>MAPAEILNGKEISAQIRARLKNQVTQLKEQVPGFTPRLAILQVGNRDDSNLYINVKLKAAEEIGIKATHIKLPRTTTESEVMKYITSLNEDSTVHGFLVQLPLDSENSINTEEVINAIAPEKDVDGLTSINAGRLARGDLNDCFIPCTPKGCLELIKETGVPIAGRHAVVVGRSKIVGAPMHDLLLWNNATVTTCHSKTAHLDEEVNKGDILVVATGQPEMVKGEWIKPGAIVIDCGINYVPDDKKPNGRKVVGDVAYDEAKERASFITPVPGGVGPMTVAMLMQSTVESAKRFLEKFKPGLEHHHHHH[4x]

Methylenetetrahydrofolate dehydrogenase/cyclohydrolase 2 (MTHFD2) is a bifunctional metabolic enzyme found in mitochondria, exhibiting both dehydrogenase and cyclohydrolase catalytic activities. In one-carbon metabolism, MTHFD2 converts 5, 10-methylene tetrahydrofolate (5,10-CH2-THF) to 10-formyl tetrahydrofolate (10-CHO-THF) in mitochondria, thereby regulating the production of NADH, purines, and pyrimidines. An isozyme, methylenetetrahydrofolate dehydrogenase, cyclohydrolase and formyltetrahydrofolate synthetase 1 (MTHFD1), performs similar catalytic reactions to MTHFD2, albeit localized in the cytoplasm rather than the mitochondrion. The key distinction between these two proteins lie in their expression profiles: MTHFD1 is typically expressed in normal cells while MTHFD2 is abundantly expressed in immortal, embryonic, and cancer cells, but absent in adult normal cells.

Superimposition of the MTHFD1/16e complex structure with MTHFD1/LY374571 complex structure uncovered several differences between them. First, in the structure of MTHFD1/LY374571, the nicotinamide group of NADP+ was hydrogen bonded with the NH2 moiety of the triaminopyrimidine headgroup of LY374571. However, the addition of a chloride substituent on the phenyl ring in 16e induced a clash with the nicotinamide group of NADP+, leading to the shift of the nicotinamide group of NADP+ away from the triaminopyrimidine headgroup of 16e and the consequent loss of the hydrogen bond between 16e and NADP+ Instead, NADP+ in MTHFD1/16e structure was found to be hydrogen bonded with the side chain of Thr279. Second, in comparison with the MTHFD1/LY374571 structure, it was observed that the addition of the chloride atom in 16e led to the rotation of the phenyl ring by approximately 26°, accompanied by the movement of the γ-carboxylic acid away from β strand h1. Moreover, the electron density of the γ-carboxylic acid in 16e is weaker than that observed in LY374571. The shift of γ-carboxylic acid in 16e resulted in the loss of the van der Waals interactions with Leu51, Tyr52 and Tyr240. These effects collectively contributed to the weaker inhibitory activity of 16e toward MTHFD1 and consequently improved its selectivity to MTHFD2, as shown by the increase in the selectivity index from 7.9 to 27.1 compared with LY374571. The γ-carboxylic acid of 16e adopted different conformations in MTHFD1 and MTHFD2. In the MTHFD2/16e structure, the γ-carboxylic acid was positioned toward β strand h1, forming hydrogen bonds with Ser83 and hydrophobic interactions with Tyr84 and Leu289. However, in the MTHFD1/16e structure, the γ-carboxylic acid moiety shifted away, leading to the loss of these interactions.> MHHHHHHSETSRTAFGGRRAVPPNNSNAAEDDLPTVELQGVVPRGVNLQEFLNVTSVHLFKERWDTNKVDHHTDKYENNKLIVRRGQSFYVQIDFSRPYDPRRDLFRVEYVIGRYPQENKGTYIPVPIVSELQSGKWGAKIVMREDRSVRLSIQSSPKCIVGKFRMYVAVWTPYGVLRTSRNPETDTYILFNPWCEDDAVYLDNEK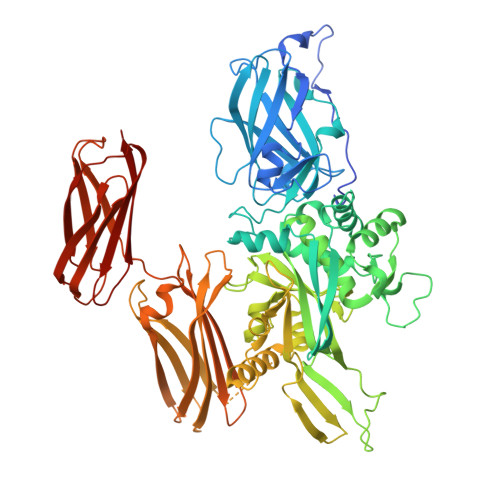EREEYVLNDIGVIFYGEVNDIKTRSWSYGQFEDGILDTCLYVMDRAQMDLSGRGNPIKVSRVGSAMVNAKDDEGVLVGSWDNIYAYGVPPSAWTGSVDILLEYRSSENPVRYGQCWVFAGVFNTFLRCLGIPARIVTNYFSAHDNDANLQMDIFLEEDGNVNSKLTKDSVWNYHCWNEAWMTRPDLPVGFGGWQAVDSTPQENSDGMYRCGPASVQAIKHGHVCFQFDAPFVFAEVNSDLIYITAKKDGTHVVENVDATHIGKLIVTKQIGGDGMMDITDTYKFQEGQEEERLALETALMYGAKKPLNTEGVMKSRSNVDMDFEVENAVLGKDFKLSITFRNNSHNRYTITAYLSANITFYTGVPKAEFKKETFDVTLEPLSFKKEAVLIQAGEYMGQLLEQASLHFFVTARINETRDVLAKQKSTVLTIPEIIIKVRGTQVVGSDMTVIVEFTNPLKETLRNVWVHLDGPGVTRPMKKMFREIRPNSTVQWEEVCRPWVSGHRKLIASMSSDSLRHVYGELDVQIQRRPSM> SNSASSCHRPLLIPPVRPVGPGRALLL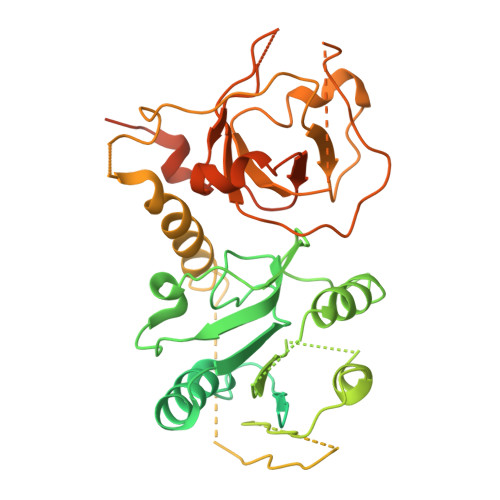LPVEQGFTFSGICRVTCLYGQVQVFGFTISQGQPAQDIFSVYTHSCLSIHALHYSQPEKSKKELKREARNLLKSHLNLDDRRWSMQNFSPQCSIVLLEHLKTATVNFITSYPGSSYIFVQESPTPQIKPEYLALRSVGIRREKKRKGLQLTESTLSALEELVNVSCEEVDGCPVILVCGSQDVGKSTFNRYLINHLLNSLPCVDYLECDLGQTEFTPPGCISLLNITEPVLGPPFTHLRTPQKMVYYGKPSCKNNYENYIDIVKYVFSAYKRESPLIVNTMGWVSDQGLLLLIDLIRLLSPSHVVQFRSDHSKYMPDLTPQYVDDMDGLYTKSKTKMRNRRFRLAAFADALEFADEEKESPVEFTGHKLIGVYTDFAFRITPRNRESHNKILRDLSILSYLSQLQPPMPKPLSPLHSLTPYQVPFNAVALRITHSDVAPTHILYAVNASWVGLCKIQDDVRGYTNGPILLAQTPICDCLGFGICRGIDMEKRLYHILTPVPPEELRTVNCLLVGAIAIPHCVLKCQRGIEGTVPYVTTDYNFKLPGASEKIGAREPEEAHKEKPYRRPKFCRKMK>[3x]MTNIAKAQPKLYVMDNGRMRMDKNWMIAMHNPATIANPNAPTEFIEFPIYTVLIDHPEGKILFDTSCNPDSMGAQGRWGEATQSMFPWTASEECYLHNRLEQLKVRPEDIKFVIASHLHLDHAGCLEMFTNATIIVHEDEFSGALQTYARNQTEGAYIWGDIDAWIKNNLNWRTIKRDEDNIVLAEGIKILNFGSGHAWGMLGLHVQLPEKGGIILASD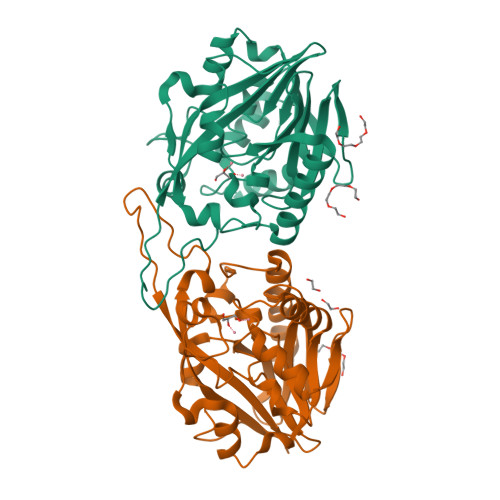AVYSAESYGPPIKPPGIIYDSLGFVRSVEKIKRIAKETNSEVWFGHDSEQFKRFRKSTEGYYE>[3x]ASNFTQFVLVDNGGTGDVTVAPSNFANGVAEWISSNSRSQAYKVTCSVRQSSAQNRKYTIKVEVPKVATQTVGGVELPVAAWRSYLSM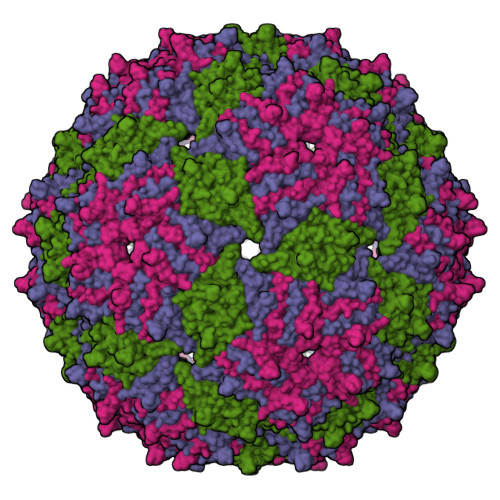KLTIPIFATNSDCELIVKAMQGLLKDGNPIPSAIAANSGIY>PGSIPLIGERFPEMEVTTDHGVIKLPDHYVSQGKWFVLFSHPADFTPVSTTEFVSFARRYEDFQRLGVDLIGLSVDSVFSHIKWKEWIERHIGVRIPFPIIADPQGTVARRLGLLHAESATHTVRGVFIVDARGVIRTMLYYPMELGRLVDEILRIVKALKLGDSLKRAVPADWPNNEIIGEGLIVPPPTTEDQARARMESGQYRCLDWWFCWDTPASRDDVEEA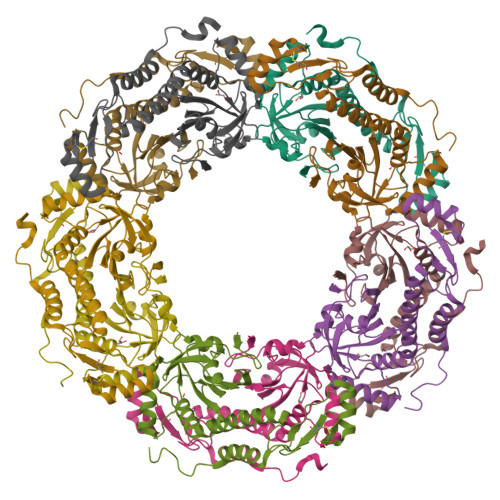RRYLRRAAEKPAKLLYEEARTHLH[10x]>MHHHHHHSGENLYFQSMKQTYMIVNELDVNKGGMTTAMLTRSKFFLDNEISGDIITFDFKANYKDILKELVQSKKMDKRTQMHNPFIYFKNISNLQHKKYNYTMTRNLSNLLKDSVEIKENSRISRFFNIMSREYLAYKRETEQETIFDLFKNNLRYKRIYFYKGKIVKTEVFNSDNNLIAEQFYDDNGYLYLYRQINPEKKSIGKTYLVCKEKQFKNNVEFCSYFLDKLIPDINDNIIICDGPGSFPKILKTNHKNVKKFAVIHVNHYKNFDDTGAVKKQEDYILRNANKINGVVMLTEAQKKDIIEKYKITNAYVISNFINITDDYRDKNDNKVVGHISRLVPQKGLPYLIDVAKKVVEQDNSVEFHLYGTGEEKSKIENLIQESNLTNNVKLLGYTTNAIEKIKDFRCVISTSQFEGQGLSLIEAMLLKKPVVAFDVKYGPSDFVKDGKNGYLIENKDIKKMANKILKLLHDKELSKSLGKHGRDTIIDMYQPEKLMVKWKQLFN[4x]

Staphylococcus epidermidis expresses glycerol phosphate wall teichoic acid (WTA), but some health care–associated methicillin-resistant S. epidermidis (HA-MRSE) clones produce a second, ribitol phosphate (RboP) WTA, resembling that of the aggressive pathogen Staphylococcus aureus. We report here that the TarM enzyme of HA-MRSE [TarM(Se)] glycosylates RboP-WTA with glucose, instead of N-acetylglucosamine (GlcNAc) by TarM(Sa) in S. aureus. Each blade of the homotrimer contains a catalytic domain with a canonical GT-B fold, consisting of an N-terminal acceptor substrate-binding domain (ABD; residues 1 to 68 and 202 to 302) and a C-terminal nucleotide-binding domain (residues 303 to 492). TarM(Se) is a retaining WTA glycosyltransferase; therefore, the relative positions of donor and acceptor substrates in TarM(Se) and TarP are different.

Extensive structural characterization of TarM(Se)G117R with donor and acceptor substrates, in particular, with product uridine diphosphate (UDP) and glycosylated poly(RboP) explains the binding mode of poly(RboP) and the catalytic mechanism of a retaining WTA glycosyltransferase. In the initial refinement, we noticed a disc-shaped, strong positive difference electron density that connected to C4 hydroxyl of RboP2 in all four copies of the TarM(Se)G117R ternary complex in the asymmetric unit. We used 4RboP-glucose instead of 4RboP, did further refinement, and concluded that our ternary structure represents a complex of TarM(Se)G117R with product UDP and glycosylated 4RboP that carries a glucose residue at the C4 position of RboP2 (4RboP-glucose). Four interactions for the phosphate group of RboP2 in the binary structure are present in the ternary complex structure, while the ribitol moiety of RboP2 contacts the side chain of Glu10, and the glucose at C4 position is hydrogen-bonded to the Gln265 side chain. The phosphate group of RboP3 is fixed by two tandem backbone amide groups of Gly16, Gly17, Met18, and Thr19, and its ribitol moiety is hydrogen-bonded to the side chains of Arg326 and Gln330. The key interactions between TarM(Se)G117R and 4RboP-glucose are formed mainly by backbone amide groups that serve to anchor phosphate groups of 4RboP-glucose into the P1, P2, and P3 sites, while Arg326 and Gln330 side chains interact with the ribitol moiety of RboP3, with help from Lys263 and Asn255, leading the poly(RboP) fragment to adopt a V-shaped conformation, in which the phosphate group of RboP3 is located at the vertex. As a result of these interactions, 4RboP-glucose rests in an extended electropositive groove on the TarM(Se) surface. The observed geometry and distances nicely support an internal nucleophilic substitution (SNi)-like mechanism. The ternary complex structure of TarM(Se)G117R bound to UDP and 4RboP-glucose provides, for the first time, clear evidence that a glycosyltransferase glycosylates WTA in a processive manner.>[3x]MKLIFAIVQDQDSNRLSDALTKG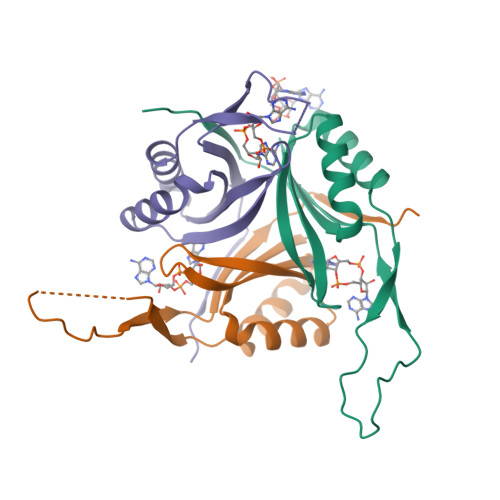NFGATKLATTGGFLKAGNTTFIIGTEDERVEDALAIIKENCKAREQMMTPSASLGVTVDTYVPYPIEVQVGGATVFVMPVESFHHFLEHH CarD, first identified as a regulator of ribosomal RNA (rRNA) transcription in Mycobacterium tuberculosis (Mtb), is a transcriptional activator widely distributed among bacterial species, including Thermus species, but is absent in Eco. CarD is a global regulator that is an essential protein in Mtb, the causative agent of tuberculosis. Crystal structures of Tth and Mtb CarD reveal an N-terminal domain with a Tudor-like fold (CarD-RID, RNAP interacting domain) in common with the Eco transcription repair coupling factor (TRCF)-RID, and a helical C-terminal domain (CarD-CTD). The structural results, combined with supporting biochemical studies, establish that the CarD-RID makes a protein/protein interaction with the RNAP β1-lobe, thereby positioning the CarD-CTD and a conserved Trp residue to interact with the upstream edge of the transcription bubble, using a wedge mechanism to prevent collapse of the transcription bubble.

Docking CarD onto the RNAP was facilitated by a high-resolution crystal structure of a Tth CarD/Taq β1-lobe complex (2.4 Å-resolution). Unique among known transcription activators, the CarD-RID interacts with the RNAP β subunit β1-lobe (corresponding to the eukaryotic RNAP II Rpb2 protrusion domain; Cramer et al., 2001), which is near the upstream portion of the transcription bubble in RPo. The relative orientation of the CarD domains (CarD-RID, CarD-CTD) seen in the Thermus CarD and CarD/β1-lobe structures is only slightly altered in the Thermus CarD/RPo complex: the CarD-CTD is rotated ∼11° (with respect to the CarD-RID) to interact with the DNA. By maintaining the CarD-RID/CTD interface seen in all the Tth CarD structures, binding of the CarD-RID to the RNAP β1-lobe positions the CarD-CTD to interact directly with the upstream ds/ss junction of the transcription bubble. A crystal structure of Mtb CarD in complex with an Mtb RNAP β-subunit fragment that includes the β1-lobe shows a relative orientation of the CarD-RID/CarD-CTD domains very different from the one in our Tth CarD structures, despite high sequence and structural similarity within the domains. In the Mtb structure, the CarD-CTD is rotated ∼140° relative to the CarD-RID.

> PLTEIQVESYKKALQADVPPEKRENVGIQAAFKETFPIEEGDKGKGGLVLDFLEYRIGDPPFSQDECREKDLTYQAPLYARLQLIHKDTGLIKEDEVFLGHLPLMTEDGSFIINGADRVIVSQGGRTVGELMADQFRVGLARLARGVRERMVMGSPDTLTPAKLVNSRPLEAALREFFSRSQLS;> EFRPGDKVVLPPYGVGVVAGIAQRSVSGVSRAYYQVDFPGSRSKAYVPVEAPHSVGLRKALAPEEVPVILDLLKNGRMPLPKQWAARHRKTSEILADGNPYRIAQMAGQLRAWEVERGLPDLDRQALRRAIHLLAEEVAQSLEITVQEAKRLFEEAWG> MTERPSLSPREARDRYLAHRQTDAADASIKSFRYRLKHFVEWAEERDITAMRELTGWKLDEYETFRRGSDVSPATLNGEMQTLKNWLEYLARIDVVDEDLPEKVHV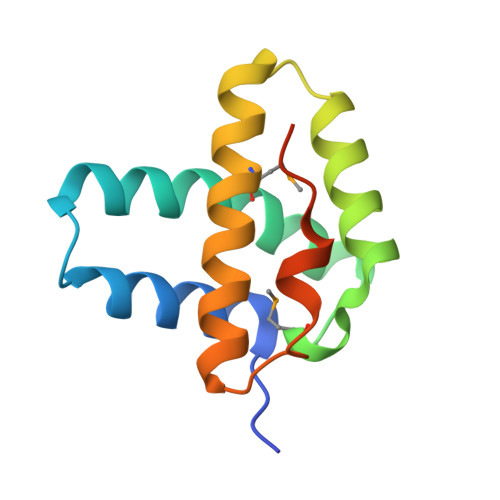PTILEHHHHHH> AASMSVQAEIGILDHVDGSSEFVSQDTKVICSVTGPIEPKARQELPTQLALEIIVRPAKGVATTREKVLEDKLRAVLTPLITRHCYPRQLCQITCQILESGEDEAEFSLRELSCCINAAFLALVDAGIALNSMCASI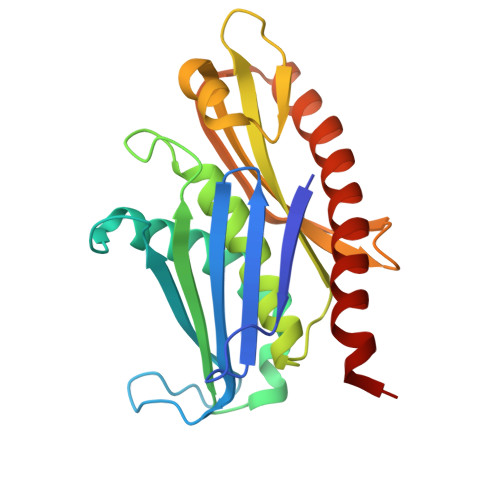PIAIIKDTSDIIVDPTAEQLKISLSVHTLALEFVNGGKVVKNVLLLDSNGDFNEDQLFSLLELGEQKCQELVTNIRRIIQDNISPRLVV In order to understand the structural basis for the effect of N6‐methyladenine on k‐turn conformation, we have used X‐ray crystallography to investigate the structural effect of this modification on different base pairs involving adenine. Each species was formed by the hybridization of a self‐complementary strand that contains a 5‐bromocytosine nucleotide used to calculate phases for the diffraction in most cases. Crystallography reveals that N6‐methylation of adenine prevents the formation of trans Hoogsteen‐sugar A·G base pairs, explaining why the box C/D RNA cannot adopt its kinked conformation. More generally, our data indicate that sheared A·G base pairs (but not Watson–Crick base pairs) are more susceptible to disruption by N6mA methylation and are therefore possible regulatory sites.

The RNA duplex adopts standard A‐form helical geometry and the N6mA‐U base pairs are normal Watson–Crick pairs. Formation of the cis Watson–Crick base pair requires that the N6‐methyl adopts an anti geometry to allow conventional basepairing with H‐bonding from AN6 to UO4. We have shown that the Watson–Crick base pairs A‐U and A‐G can form normally despite methylation of adenine at N6, although the A‐U base pair has been shown to be destabilized to some degree 43.

>GGACUAGUCC[4x]> LPSPSRQA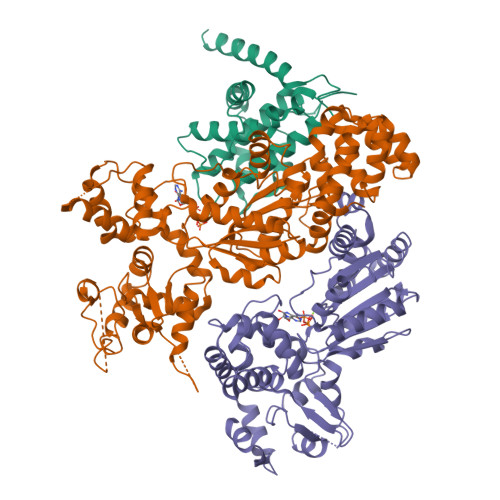STRRMSIGESIDGKINDWEEPRLDIEGFVVDYFTHRIRQNGMEWFGAPGLPSGVQPEHEMMRVMGTIFEKKHAENFETFSEQLLAVPRISFSLYQDVVRTVGNAQTDQSPMSYGRLIGLISFGGFVAAKMMESVELQGQVRNLFVYTSLFIKTRIRNNWKEHNRSWDDFMTLGKQMKEDYERAEAEKVGRRKQNRR;>[2x]MLCEIECRALSTAHTRLIHDFEPRDALTYLEGKNIFTEDHSELISKMSTRLERIANFLRIYRRQASELGPLIDFFNYNNQSHLADFLEDYIDFAINEPDLLRPVVIAPQFSRQMLDRKLLLGNVPKQMTCYIREYHVDRVIKKLDEMCDLDSFFLFLHGRAGSGKSVIASQALSKSDQLIGINYDSIVWLKDSGTAPKSTFDLFTDILLMLKSEDDLLNFPSVEHVTSVVLKRMICNALIDRPNTLFVFDDVVQEETIRWAQELRLRCLVTTRDVEISNAASQTCEFIEVTSLEIDECYDFLEAYGMPMPVGEKEEDVLNKTIELSSGNPATLMMFFKSCEPKTFEKMAQLNNKLESRGLVGVECITPYSYKSLAMALQRCVEVLSDEDRSALAFAVVMPPGVDIPVKLWSCVIPVDICSNEEEQLDDEVADRLKRLSKRGALLSGKRMPVLTFKIDHIIHMFLKHVVDAQTIANGISILEQRLLEIGNNNVSVPERHIPSHFQKFRRSSASEMYPKTTEETVIRPEDFPKFMQLHQKFYDSLKNFACC>[2x]CPRFLKVKNWETDVVLTDTLHLKSTLETGCTEHICMGSIMLPSQHTRKPEDVRTKDQLFPLAKEFLDQYYSSIKRFGSKAHMDRLEEVNKEIESTSTYQLKDTELIYGAKHAWRNASRCVGRIQWSKLQVFDARDCTTAHGMFNYICNHVKYATNKGNLRSAITIFPQRTDGKHDFRVWNSQLIRYAGYKQPDGSTLGD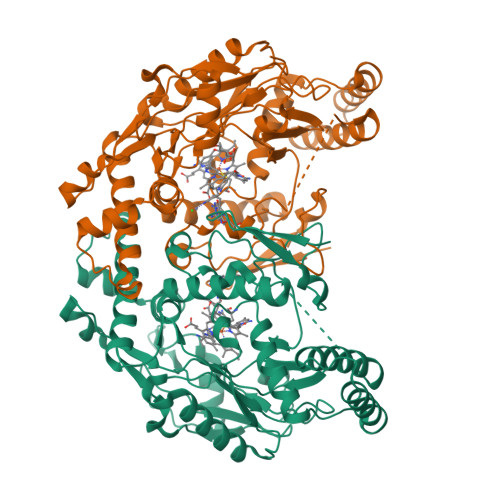PANVQFTEICIQQGWKAPRGRFDVLPLLLQANGNDPELFQIPPELVLEVPIRHPKFDWFKDLGLKWYGLPAVSNMLLEIGGLEFSACPFSGWYMGTEIGVRDYCDNHRYNILEEVAKKMDLDMRKTSSLWKDQALVEINIAVLYSFQSDKVTIVDHHSATESFIKHMENEYRCRGGCPADWVWIVPPMSGSITPVFHQEMLNYRLTPSFEYQPDPWNTHVWKG> LVVPNINSSNPTTSNSAPALDAAETGHTSSVQPEDVIETRYVQTSQTRDEMSLESFLGRSGCIHESKLEVTLANYNKENFTVWAINLQEMAQIRRKFELFTYTRFDSEITLVPCISALSQDIGHITMQYMYVPPGAPVPNSRDDYAWQSGTNASVFWQHGQAYPRFSLPFLSVASAYYMFYDGYDEQDQNYGTANTNNMGSLCSRIVTEKHIHKVHIMTRIYHKAKHVKAWCPRPPRALEYTRAHRTNFKIEDRSIQTAIVTRPIITTA;> RIIQITRGDSTITSQDVANAIVAYGVWPHYLSSKDASAIDKPSQPDTSSNRFYTLRSVTWSSSSKGWWWKLPDALKDMGIFGENMFYHYLGRSGYTIHVQCNASKFHQGTLIVALIPEHQIASALHGNVNVGYNYTHPGETGREVKAETRLNPDLQPTEEYWLNFDGTLLGNITIFPHQFINLRSNNSATIIAPYVNAVPMDSMRSHNNWSLVIIPICPLETSSAINTIPITISISPMCAEFSGARAKRQ;> GLPVFITPGSGQFLTTDDFQSPCALPWYHPTKEISIPGEVKNLVEICQVDSLVPINNTDTYINSENMYSVVLQSSINAPDKIFSIRTDVASQPLATTLIGEISSYFTHWTGSLRFSFMFCGTANTTVKLLLAYTPPGIAEPTTRKDAMLGTHVIWDVGLQSTISMVVPWISASHYRNTSPGRSTSGYITCWYQTRLVIPPQTPPTARLLCFVSGCKDFCLRMARDTNLHLQSGAIAQ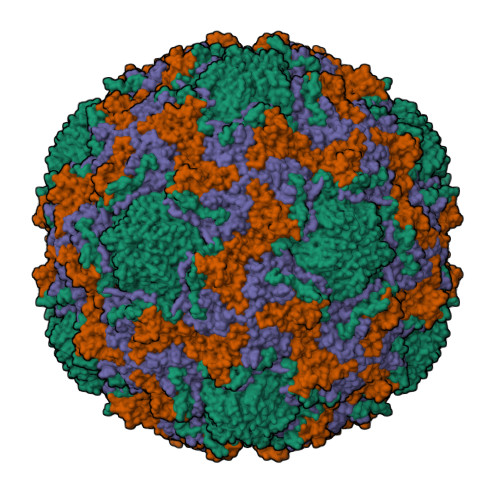;> AQVSRQNYFNINYFKDAASNGASKL> LVKEEIQAKEYLENLNKELAKRTNVETEAAWAYGSNITDENEKKKNEISAELAKFMKEVASDTTKFQWRSYQSEDLKRQFKALTKLGYAALPEDDYAELLDTLSAMESNFAKVKVCDYKDSTKCDLALDPEIEEVISKSRDHEELAYYWREFYDKAGTAVRSQFERYVELNTKAAKLNNFTSGAEAWLDEYEDDTFEQQLEDIFADIRPLYQQIHGYVRFRLRKHYGDAVVSETGPIPMHLLGNMWAQQWSEIADIVSPFPEKPLVDVSAEMEKQGYTPLKMFQMGDDFFTSMNLTKLPQDFWDKSIIEKPTDGRDLVCHASAWDFYLIDDVRIKQCTRVTQDQLFTVHHELGHIQYFLQYQHQPFVYRTGANPGFHEAVGDVLSLSVSTPKHLEKIGLLKDYVRDDEARINQLFLTALDKIVFLPFAFTMDKYRWSLFRGEVDKANWNCAFWKLRDEYSGIEPPVVRSEKDFDAPAKYHISADVEYLRYLVSFIIQFQFYKSACIKAGQYDPDNVELPLDNCDIYGSAAAGAAFHNMLSMGASKPWPDALEAFNGERIMSGKAIAEYFEPLRVWLEAENIKNNVHIGWTTSNKCVS;>YW[2x]

Angiotensin-I-converting enzyme (ACE, EC 3.4.15.1) is a promiscuous zinc metallopeptidase with a number of substrates, including the vasoregulatory peptides angiotensin I and bradykinin, the anti-fibrotic agent N-acetyl-SDKP, the neurotransmitter substance P, and amyloid-β peptide. Here, we present the use of the Drosophila melanogaster ACE homologue, AnCE (which, in particular, shares enzymatic properties with cACE), as a model to study the structural basis of ACE inhibition. The active site is located at the centre of this channel, marked by the location of the catalytic zinc ion, which is coordinated by His367, His371, and Glu395. The high-resolution crystal structures of AnCE in complex with the dipeptides VW, IW, YW, RW, and WR presented here reveal dual binding in both the non-prime (dipeptide-1) and prime (dipeptide-2) subsites of AnCE.

The YW-1 tyrosine forms a H-bond with Tyr496, which is not possible in IW and VW; however, it maintains the hydrophobic contact with Trp341 observed with those dipeptides. In YW-2, the tyrosine side chain forms hydrophobic contacts with Ala338 and Thr364 and a H-bond with Thr364. Interestingly, YW-2 folds in a conformation that allows for a π-stacking interaction between the tyrosine and tryptophan of the dipeptide. The additional difference map density around the tyrosine side chain in the S1′ subsite resulted in alternative conformations of the side chain to be tested, as well as dual conformations with the whole dipeptide flipped. The electron density remained ambiguous; for this reason, the dipeptide was left in a singular conformation. This ambiguity could be caused by lower affinity binding displayed by the dipeptide (Ki: 0.75 mM), which, in turn, could be caused by Thr364, though forming a H-bond, it could also have a repelling effect on the aromatic ring. The YW dipeptide shows low affinity for AnCE, with a Ki value of 750 µM (0.75 mM). The less clear electron density for YW bound to AnCE could be the result of low affinity binding causing the dipeptide to have low occupancy, or it could also be an indication of the tyrosine not being completely stabilised in one conformation, potentially due to the repelling effect that Thr364 could have on the aromatic ring of the tyrosine. This effect would also be present in nACE but not in cACE, which has a valine instead. The substitution to Phe512 in cACE could influence the binding of YW-1, as this would remove the possibility of the H-bond within this region, and instead be replaced with potential hydrophobic interactions.>[4x]MFLKVRAEKRLGNFRLNVDFEMGRDYCVLLGPTGAGKSVFL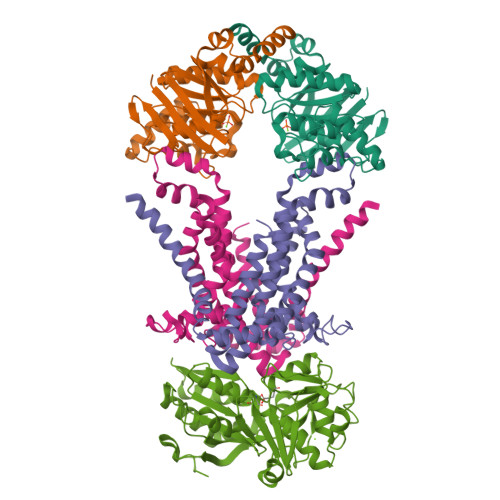ELIAGIVKPDRGEVRLNGADITPLPPERRGIGFVPQDYALFPHLSVYRNIAYGLRNVERVERDRRVREMAEKLGIAHLLDRKPARLSGGERQRVALARALVIQPRLLLLDEPLSAVDLKTKGVLMEELRFVQREFDVPILHVTHDLIEAAMLADEVAVMLNGRIVEKGKLKELFSAKNGEVAEFLSARNLLLKVSKILD;>[4x]MGHHHHHHHHHHSSGENLYFQGHMRLLFSALLALLSSIILLFVLLPVAATVTLQLFNFDEFLKAASDPAVWKVVLTTYYAALISTLIAVIFGTPLAYILARKSFPGKSVVEGIVDLPVVIPHTVAGIALLVVFGSSGLIGSFSPLKFVDALPGIVVAMLFVSVPIYINQAKEGFASVDVRLEHVARTLGSSPLRVFFTVSLPLSVRHIVAGAIMSWARGISEFGAVVVIAYYPMIAPTLIYERYLSEGLSAAMPVAAILILLSLAVFVALRIIVGREDVSEGQG;>GHMNVKLKVFHAGSLTEPMKAFKRAFEEKHPNVEVQTEAAGSAATIRKVTELGRKADVIATADYTLIQKMMYPEFANWTIMFAKNQIVLAYRNDSRYADEINSQNWYEILKRPDVRFGFSNPNDDPCGYRSLMAIQLAELYYNDPTIFDELVAKNSNLRFSEDNGSYVLRMPSSERIEINKSKIMIRSMEMELIHLVESGELDYFFIYKSVAKQHGFNFVELPVEIDLSSPDYAELYSKVKVVLANGKEVTGKPIVYGITIPKNAENRELAVEFVKLVISEEGQEILRELGQEPLVPPRADTAVPSLKAMVEVS[2x]(2R)-2-[(1S,2R)-1-carboxy-2-hydroxypropyl]-5-[(2R)-oxolan-2-yl]-2,3-dihydro-1,3-thiazole-4-carboxylic 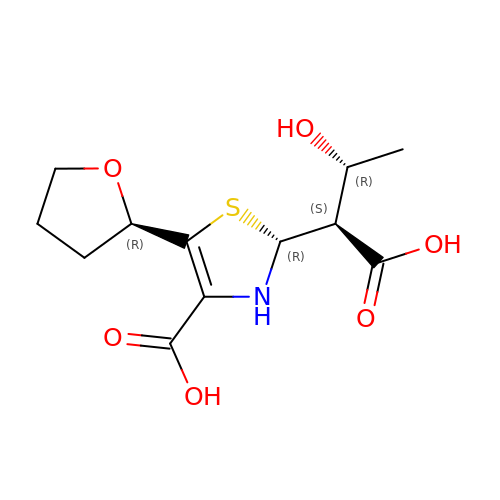acid | C12 H17 N O6 S | CGJDLFMMMJEANA-DAGMQNCNSA-N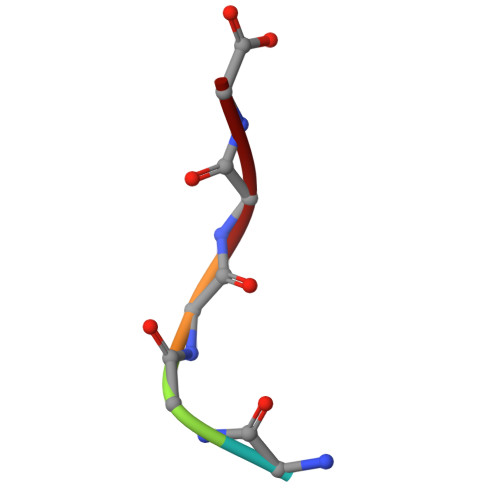> GGGGG> MPSALAIFTCRPNSHPFQERHVYLDEPIKIGRSVARCRPAQNNATFDCKVLSRNHALVWFDHKTGKFYLQDTK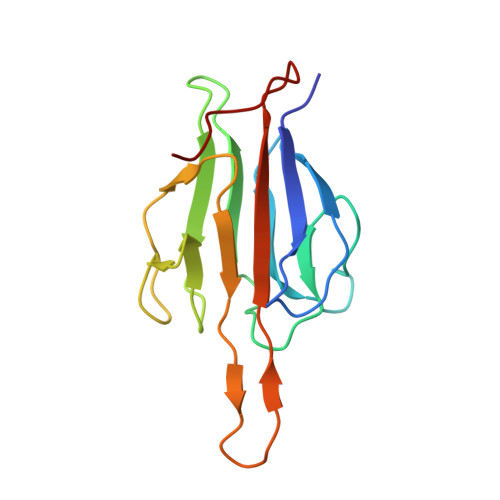SSNGTFINSQRLSRGSEESPPCEILSGDIIQFGVDVTENTRKVTHGCIVSTIKLFLPDGMEARLRSD> 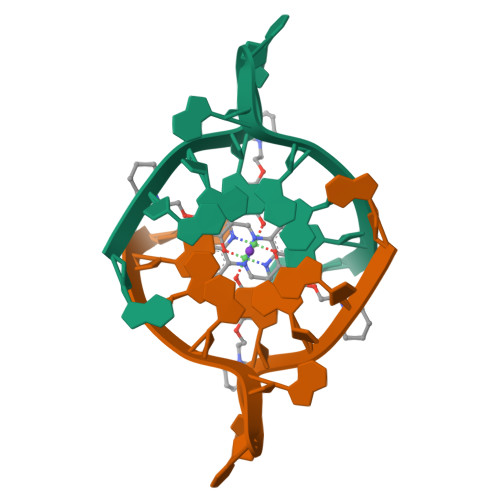AGGGTTAGGGTT>[2x]MSAIFAERALLPEGWARNVRFEISADGVLAEIRPDANADGAERLGGAVLPGMPNLHSHAFQRAMAGLAEVAGNPNDSFWTWRELMYRMVARLSPEQIEVI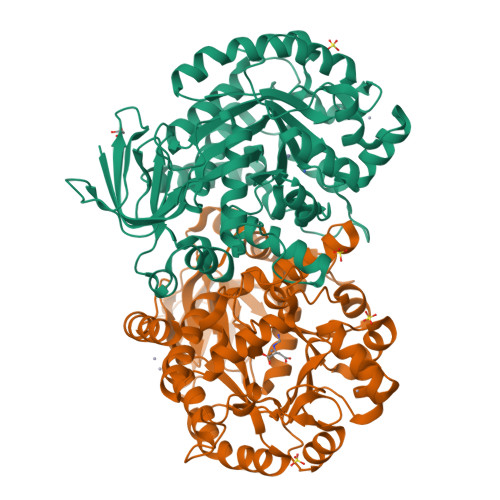ACQLYIEMLKAGYTAVAEFHYVHHDLDGRSYADPAELSLRISRAASAAGIGLTLLPVLYSHAGFGGQPASEGQRRFINGSEAYLELLQRLRAPLEAAGHSLGLCFHSLRAVTPQQIATVLAAGHDDLPVHIHIAEQQKEVDDCQAWSGRRPLQWLYENVAVDQRWCLVHATHADPAEVAAMARSGAVAGLCLSTEANLGDGIFPATDFLAQGGRLGIGSDSHVSLSVVEELRWLEYGQRLRDRKRNRLYRDDQPMIGRTLYDAALAGGAQALGQPIGSLAVGRRADLLVLDGNDPYLASAEGDALLNRWLFAGGDRQVRDVMVAGRWVVRDGRHAGEERSARAFVQVLGELLD> MNDHIHRVPALTEEEIDSVAIKTFERYALPSSSSVKRKGKGVTILWFRNDLRVLDNDALYKAWSSSDTILPVYCLD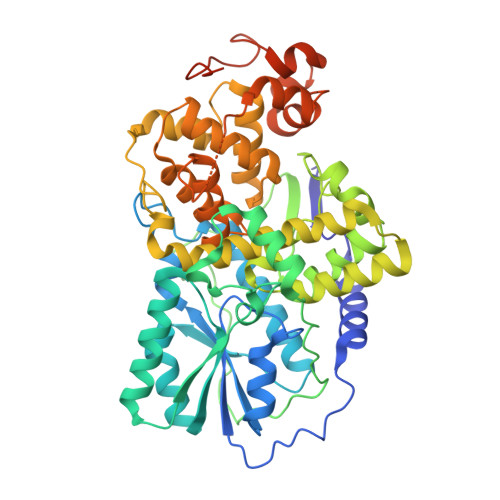PRLFHTTHFFNFPKTGALRGGFLMECLVDLRKNLMKRGLNLLIRSGKPEEILPSLAKDFGARTVFAHKETCSEEVDVERLVNQGLKRVGNSTKLELIWGSTMYHKDDLPFDVFDLPDVYTQFRKSVEAKCSIRSSTRIPLSLGPTPSVDDWGDVPTLEKLGVEPQEVTRGMRFVGGESAGVGRVFEYFWKKDLLKVYKETRNGMLGPDYSTKFSPWLAFGCISPRFIYEEVQRYEKERVANNSTYWVLFELIWRDYFRFLSIKCGNSLFHLGGPRNVNGKWSQDQKLFESWRDAKTGYPLIDANMKELSTTGFMSNRGRQIVCSFLVRDMGLDWRMGAEWFETCLLDYDPCSNYGNWTYGAGVNDPREDRYFSIPKQAQNYDPEGEYVAFWLQQLRRLPKEKRHWPGRLMYMDTVVPLKHGNGPMAGGSKSGGGFRGSHSGRRSRHNGP>GPRMAFTNYSSLNRAQLTFEYLHTNSTTHEFLFGALAELVDNARDADATRIDIYAERREDLRGGFMLCFLDDGAGMDPSDAASVIQFGKSAKRTPESTQIGQYGNGLKSGS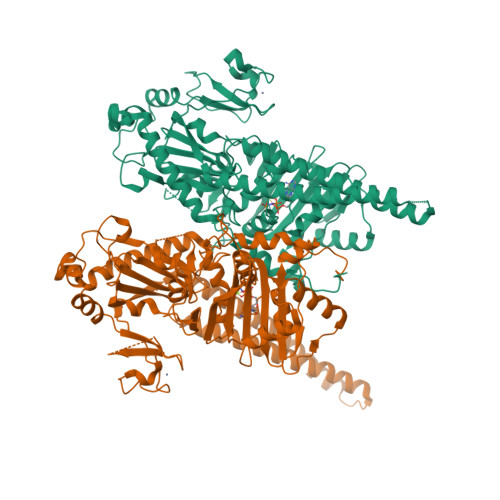MRIGKDFILFTKKEDTMTCLFLSRTFHEEEGIDEVIVPLPTWNARTREPVTDNVEKFAIETELIYKYSPFRTEEEVMTQFMKIPGDSGTLVIIFNLKLMDNGEPELDIISNPRDIQMAETSPEGTKPERRSFRAYAAVLYIDPRMRIFIHGHKVQTKRLSCCLYKPRMYKYTSSRFKTRAEQEVKKAEHVARIAEEKAREAESKARTLEVRLGGDLTRDSRVMLRQVQNRAITLRREADVKKRIKEAKQRALKEPKELNFVFGVNIEHRDLDGMFIYNCSRLIKMYEKVGPQLEGGMACGGVVGVVDVPYLVLEPRHNKQDFADAKEYRHLLRAMGEHLAQYWKDIAIAQRGIIKFWDEFGYLSANWNQPPSSELRYKRRRAMEIPTTIQCDLCLKWRTLPFQLSSVEKDYPDTWVCSMNPDPEQDRCEASEQKQKVPLGTFRKDMKTQEEKQKQLTEKIRQQQEKLEALQKTTPIRSQADLKKLPLEVTTRPST[2x]>[4x]ADSDVPNDILEEQLYNSVVVADYDSAVEKSKHLYEEKKSEVITNVVNKLIRNNKMNCMEYAYQLWLQGSKDIV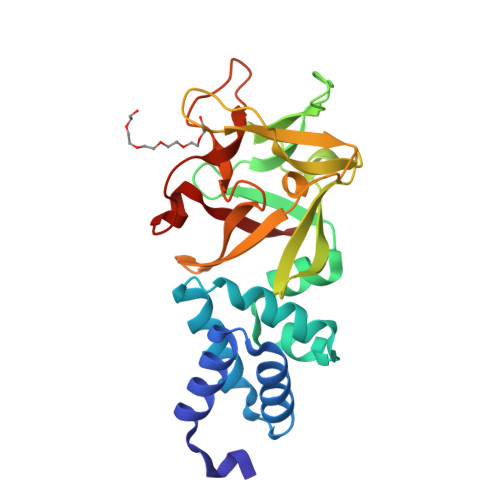RDCFPVEFRLIFAENAIKLMYKRDGLALTLSNDVQGDDGRPAYGDGKDKTSPRVSWKLIALWENNKVYFKILNTERNQYLVLGVGTNWNGDHMAFGVNSVDSFRAQWYLQPAKYDNDVLFYIYNREYSKALTLSRTVEPSGHRMAWGYNGRVIGSPEHYAWGIKAF methyl 4-(2-{5-[(3aS,4S,6aR)-2-oxo-hexahydro-1H- thieno[3,4-d]imidazolidin-4-yl]pentanehydrazido}-3- 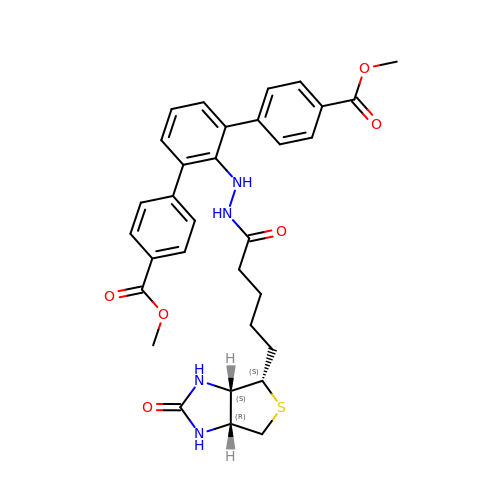[4-(methoxycarbonyl)phenyl]phenyl)benzoate | C32 H34 N4 O6 S | LVYKNIDQFONGOK-ZEZDXWPOSA-N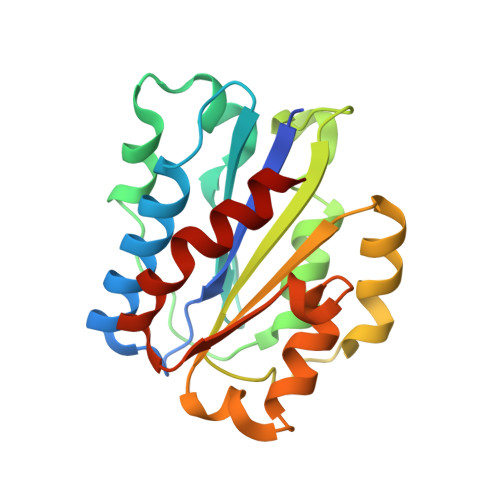> GSHMASRQEQDIVFLIDGSGSISSRNFATMMNFVRAVISQFQRPSTQFSLMQFSNKFQTHFTFEEFRRSSNPLSLLASVHQLQGFTYTATAIQNVVHRLFHASYGARRDAAKILIVITDGKKEGDSLDYKDVIPMADAAGIIRYAIGVGLAFQNRNSWKELNDIASKPSQEHIFKVEDFDALKDIQNQLKEKIFAIEG> NYKPTPWTRADALKVHSDDPTTTQPLVDVAFPVMSEEVFIWDTMPLRDFDGDIVSVNGWCVIFTLTADRNTNNPDFQDENGNYDIKRDWEDRHGRARICYWYSRTGKDWIFGGRVMAEGVSPTTREWAGTPILLNDEG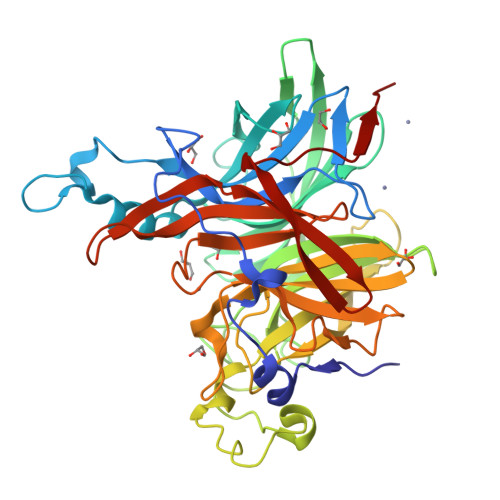DIDLYYTCVTPGATIAKVRGKIVTSDEGVSLEGFQHVKSLFSADGKIYQTEEQNAYWNFRDPSPFIDKNDGKLYMLFEGNVAGSRGTHEITQEDMGSVPPGYENVGGARYQVGCIGLAVAKDLSGDEWEILPPLITAVGVNDQTERPHFVFQEGKYYLFTISHKYTFADNLTGPDGVYGFVSNQLTGPYTPMNSSGLVLGNPSSQPFQTYSHYVMPNGLVTSFIDSVPWEGEKFRIGGTEAPTVKILLKGDRSFVVDSFDYGYIPAMKDIILK> 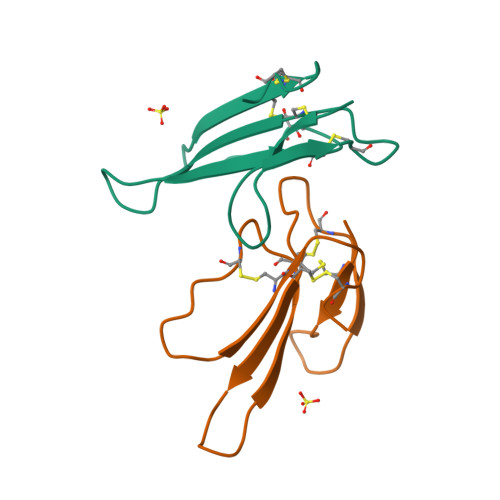LTCVTTKSIGGVTTEDCPAGQNVCFKRWHYVTPKNYDIIKGCAATCPKVDNNDPIRCCGTDKCND VACV protein A49 prevents translocation of NF-κB to the nucleus by sequestering cellular β-TrCP, a protein required for the degradation of the inhibitor of κB. Unexpectedly, the structure showed that A49 possesses a Bcl-2-like fold despite not sharing sequence identity with known cellular or poxvirus Bcl-2 family proteins. Strikingly, despite a lack of sequence conservation with known family members, A49 adopts the Bcl-2 family protein fold comprising five α-helices wrapped around a central helix, α5 (45). The A49 structure shows that A49 lacks a surface groove compatible with binding BH3 peptides and is unable to bind the proapoptotic proteins Bax or Bak.

Crystallization trials of full-length VACV A49 yielded just two crystals in a single crystallization condition after 4 months of equilibration. Diffraction data were recorded to 3.0 Å resolution (full-length A49) but, because A49 does not share identifiable sequence similarity with any proteins of known structure, it was not possible to solve the structure by molecular replacement, and repeated attempts to reproduce these crystals were unsuccessful, frustrating attempts to solve the structure by experimental methods. The structure of full-length A49 closely resembles that of the truncated protein, superposing on A49 Δ12 with 0.50–0.67 Å root mean square deviation across 140 Cα atoms. In the full-length structure, residues 1–17 could not be modeled due to a lack of interpretable electron density N-terminal to residue 18. It is possible that these amino acids were removed by serendipitous in-drop proteolysis prior to crystallization. The only other significant difference between the structures of full-length and Δ12 A49 is the conformation of the region linking helices α2 and α3, helix α3 being one turn shorter in the full-length structure. In four of the eight molecules of A49 Δ12 grown in the ammonium sulfate condition and both molecules of A49 Δ12 grown in the sodium malonate condition, a single residue (Gly) of the C-terminal purification tag is observed; in the structure of full-length A49, the final two residues (161 and 162) and the purification tag were not ordered and could not be modeled. Visual inspection of the structures of A49 Δ12 and full-length A49 showed that, in all cases, two molecules of A49 self-associate via an interaction of helices α4 and α6 (the “4-6 face”). In the structure of full-length A49 this interaction is formed by crystallographic 2-fold symmetry, whereas in the structures of A49 Δ12 the interaction is formed by pseudo-2-fold non-crystallographic symmetry. Whereas the self-association is predominantly hydrophobic in nature, in the structure of full-length A49 a symmetric salt bridge is formed at the periphery of the binding surface between the side chains of Arg136 and Asp92.

>[2x]MDEAYYSGNLESVLGYVSDMHTELASISQLVIAKIETIDNDILNKDIVNFIMCRSNLDNPFISFLDTVYTIIDQENYQTELINSLDDNEIIDCIVNKFMSFYKDNLENIVDAIITLKYIMNNPDFKTTYAEVLGSRIADIDIKQVIRENILQLSNDIRERYLKHHHHHH>GSHMCLVCSDEASGCHYGVLTCGSCKVFFKRAVEGQHNYLCAGRNDCIIDKIRRKNCPACRYRKCLQAGMNLEARKTKKKI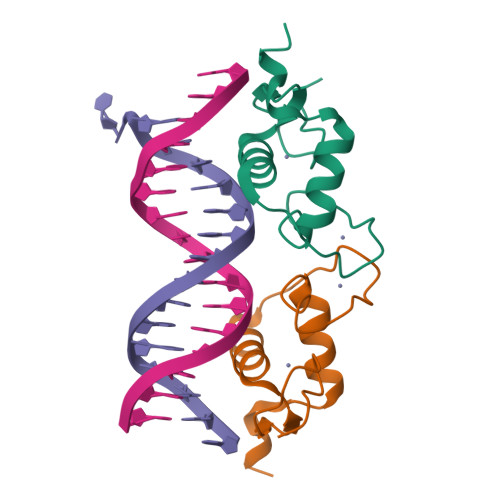KGIQQATAG[2x]> GHMQETQAVEAGEKTVEQFVQALNKGDYNKAAEMTSKKAANKSALSEKEILDKYQNIYGAADVKGLQISNLKVDKKDDS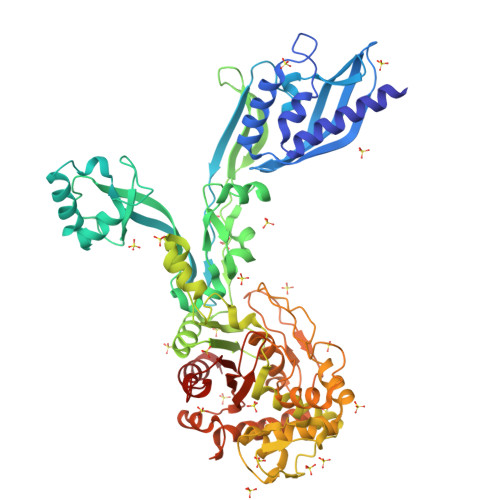TYSFSYKAKMNTSLGELKDLSYKGTLDRNDGQTTINWQPNLVFPEMEGNDKVSLTTQEAARGNIIDRNGEPLATTGKLKQLGVVPSKLGDGGEKTANIKAIASSFDLTEDAINQAISQSWVQPDYFVPLKIIDGATPELPAGATIQEVDGRYYPLGEAAAQLIGYVGDITAEDIDKNPELSSNGKIGRSGLEMAFDKDLRGTTGGKLSITDADGVEKKVLIEHEVQNGKDIKLTIDAKAQKTAFDSLGGKAGSTVATTPKTGDLLALASSPSYDPNKMTNGISQEDYKAYEENPEQPFISRFATGYAPGATFKMITAAIGLDNGTIDPNEVLTINGLKWQKDSSWGSYQVTRVSDVSQVDLKTALIYSDNIYTAQETLKMGEKKFRTGLDKFIFGEDLDLPISMNPAQISNEDSFNSDILLADTGYGQGELLINPIQQAAMYSVFANNGTLVYPKLIADKETKDKKNVIGETAVQTIVPDLREVVQDVNGTAHSLSALGIPLAAKTGTAEIKEKQDVKGKENSFLFAFNPDNQGYMMVSMLENKEDDDSATKRASELLQYLNQNYQ>[4x]MNVTIYDVAREASVSMATVSRVVNGNPNVKPSTRKKVLETIERLGYRPNAVARGLASKKTTTVGVIIPDISNIFYAELARGIEDIATMYKYNIILSNSDQNQDKELHLLNNMLGKQVDGIIFMSGNVTEEHVEELKKSPVPVVLAASIESTNQIPSVTIDYEQAAFDAVQ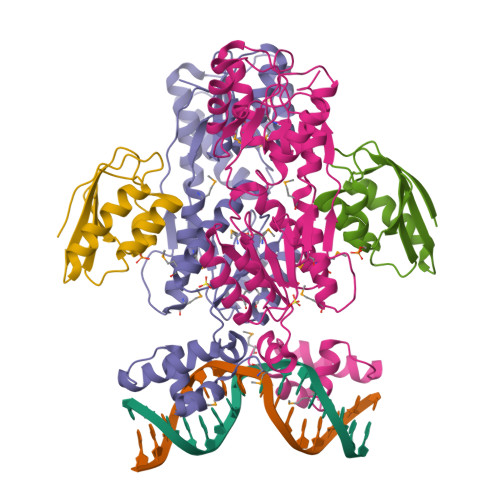SLIDSGHKNIAFVSGTLEEPINHAKKVKGYKRALTESGLPVRDSYIVEGDYTYDSGIEAVEKLLEEDEKPTAIFVGTDEMALGVIHGAQDRGLNVPNDLEIIGFDNTRLSTMVRPQLTSVVQPMYDIGAVAMRLLTKYMNKETVDSSIVQLPHRIEFRQSTK;>[4x]MAQKTFTVTADSGIHARPATTLVQAASKFDSDINLEFNGKTVNLKSIMGVMSLGIQKGATITISAEGSDEADALAALEDTMSKEGLGE> IFGIDDLIFGLLFVGFVAGGVAGGYFWGRSNGGGGGASVSSTQAGFDKIGKDIQQLRNDTNAAIEGFNGRIAHDEQAIKNLAKEIEDARAEALVGELGIIRSLIVANISMNLKESLYELANQITKRGGGIAQEAGPGCWYVDSENCDASCKEYI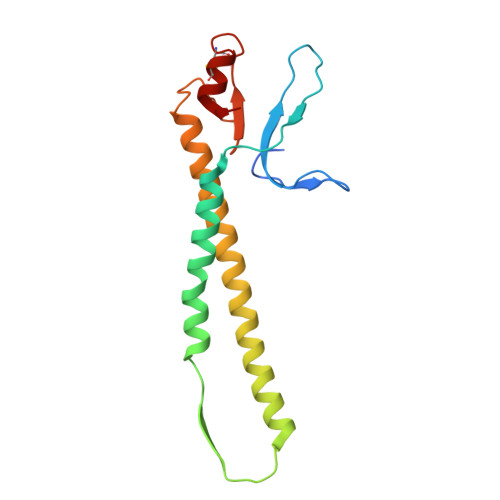FNF> MKITKLETVRVAERTNLLWVLVHTDEGITGLGETFFGAETVETYVHEYIAPRVIGRDPLQIDLLAQDLVGYLGFRSSGAEVRGNSAFDIALWDIFGKATNQPIAQLLGGFSRREIRTYNTCAGTEYIKKATGQQTANYGLSGGKDYDDLNGFLHRADELAHSLLEDGITAMKIWPFDAAAEKTRGQYISMPDLKSALEPFEKIRKAVGDKMDIMVEFHSMWQLLPAMQIAKALTPYQTFWHEDPIKMDSLSSLTRYAAVSPAPISASETLGSRWAFRDLLETGAAGVVMLDISWCGGLSEARKIASMAEAWHLPVAPHNCTGPVVLCASTHLSLNAPNALVQESVRAFYKTWYRD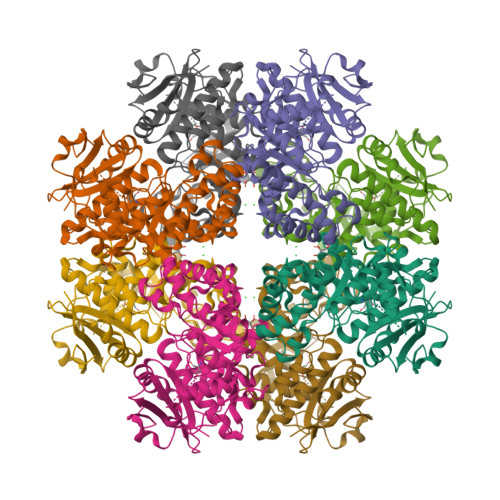LVTALPEVKNGMITVPPGAGLGMELHPDIEKTFTVSRRFSDAASI The type VI secretion system (T6SS) is a novel multi-subunit needle-like apparatus and plays an important role in many processes of bacterial life cycles, such as interspecies competition, biofilm formation and virulence-related processes. Meanwhile, to protect itself from accidental injury, the cognate immunity proteins were produced to protect the donor cells against the toxic effectors. Tae4 (type VI amidase effector 4) and Tai4 (type VI amidase immunity 4) are T6SS effector-immunity pairs from the fourth family. To this end, we determined the high-resolution crystal structure of the effector StTae4 from S. typhimurium in complex with the immunity protein EcTai4 from E. cloacae and studied the cross-neutralization of EcTai4 toward various effectors from the four families by in vitro and in vivo interactions.

The complex belonged to the P212121 space group while the Ec- and StTae4-Tai4 belonged to the C121 and P6122 space group, respectively. The results indicate that the active complex is a heterotetramer in solution, consisting of a Tai4 homodimer [named subunit I (cyan) and subunit II (orange)] binding two Tae4 molecules, consistent with the status of the Ec- and StTae4-Tai4 complexes in solution. The four heterotetramers in the asymmetric unit are likely the result of crystal packing, and represent no significant biological relevance. Clip I, composed of the residues from Gly132 to Leu142, adopts similar structure to that in the former StTae4, but a remarkable shift (∼5.4 Å) in the terminus occurs. It is worth to note that the conserved residues Cys135 and Cys139 form a disulfide bond (DSB) to stabilize the flexible loop, while there is no DSB between the two residues in the loop of the former one, where the two sulfydryl groups are in opposite directions. Moreover, the overall conformation of the Clip II in the present structure is different from that in the former one from StTae4-Tai4, which may be adaptive to the binding and inhibition of EcTai4. However, the dominant feature of the protruding loop in Tai4 is a shift by ∼3.0 Å compared with the former EcTae4, which may be adaptive for inserting into the active site of different effectors within this family. It is worth to note that the conserved residues Cys41 and Cys101, located in α2 and α5 respectively, form a DSB to stabilize the super helical conformation during the inhibition process, where there is no DSB formed between the two residues in the former EcTai4. The total buried surface area in the interface of EcTai4 dimer with one StTae4 monomer is 895 Å2, with 641 Å2 contributed by two helices (α3 and α5) from StTae4 with two helices (α3 and α4) from EcTai4 subunit I, and 254 Å2 contributed by the lid loop from StTae4 interacting with the protruding loop from the neighboring EcTai4 subunit II.

>[8x]HMASMTGGQQMGRGSMNRPSFNEAWLAFRKVNHSVADVGSIIGGNVGKNITGGYFQNACPIRMSYVLNATGFPIARNSPYAKVSGADNKFYIYRVNDMIDYLTHTMGKPDLIVNNPKQSDFIGKKGIIVVKGHGWSNARGHVTLWNGSICSDQCHLLNDPDNGPFVPEVGTLWILP;>[8x]QTLPDISTFSQQQIFENWVQNRCIGKIADSKSLKEDADASAAAWLEASNLPAENFEKADEVIVSLLKQKVGGTEPGHYQILKCTLIANSDAIRPLKSSKHHHHHH> MFLPPPECPVFEPSWEEFADPFAFIHKIRPIAEQTGICKVRPPPDWQPPFACDVDKLHFTPRIQRL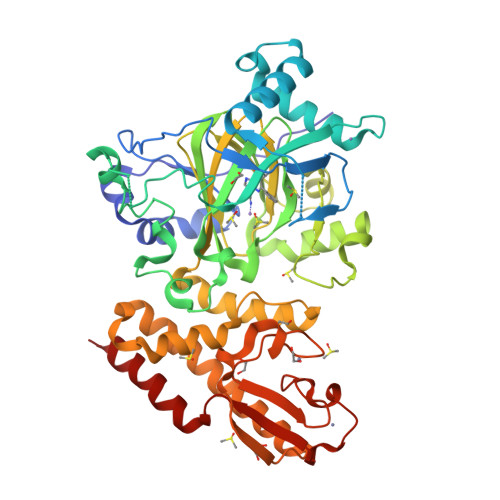NELEAQTRVKLGGGGARDYTLRTFGEMADAFKSDYFNMPVHMVPTELVEKEFWRLVSTIEEDVTVEYGADIASKEFGSGFPVRDGKIKLSPEEEEYLDSGWNLNNMPVMEQSVLAHITADICGMKLPWLYVGMCFSSFCWHIEDHWSYSINYLHWGEPKTWYGVPGYAAEQLENVMKKLAPELFVSQPDLLHQLVTIMNPNTLMTHEVPVYRTNQCAGEFVITFPRAYHSGFNQGFNFAEAVNFCTVDWLPLGRQCVEHYRLLHRYCVFSHDEMICKMASKADVLDVVVASTVQKDMAIMIEDEKALRETVRKLGVIDSERMDFELLPDDERQCVKCKTTCFMSAISCSCKPGLLVCLHHVKELCSCPPYKYKLRYRYTLDDLYPMMNALKLRAES>MNDFHRDTWAEVDLDAIYDNVENLRRLLPDDTHIMASVCGNAYGHGDVQVARTALEAGASRLAVAFLDEALALREKGIEAPILVTGASRPADAALAAQQRIALTVFRSDWLEEASALYSGPFPIHFHL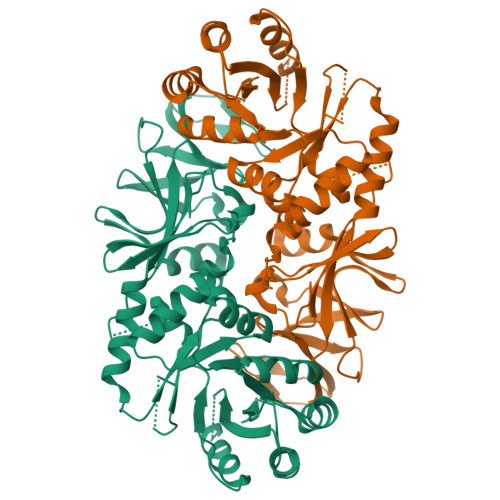YMDTGMGSLGVKDEEETKRIVALIERHPHFVLEGLWTWFATADEVNTDYFSYQYTRFLHMLEWLPSRPPLVFCANSAASLRFPDRTFNMVQFGIAMYGLAPSPGIKPLLPYPLKEAFSLHSRLVHVKKLQPGEKVSYGATYTAQTEEWIGTIPIGYKDGWLRRLQHFHVLVDGQKAPIVGRILMDMCMIRLPGPLPVGTKVTLIGRQGDKVISIDDVARHLETINYEVPCTISYRVPRIFFRHKRIMEVRNAIGRGESSAGS[3x]5,5'-di(prop-2-en-1-yl)biphenyl-2,2'-diol 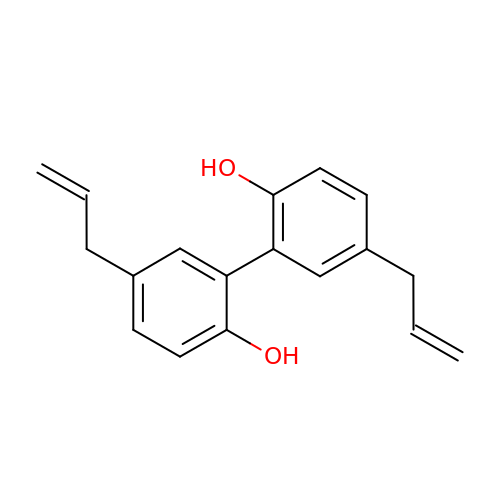| C18 H18 O2 | VVOAZFWZEDHOOU-UHFFFAOYSA-N OaPAC is a recently discovered blue-light-using flavin adenosine dinucleotide (BLUF) photoactivated adenylate cyclase from the cyanobacterium Oscillatoria acuminata that uses adenosine triphosphate and translates the light signal into the production of cyclic adenosine monophosphate. OaPAC is a homodimer of a 366-residue protein comprising an N-terminal BLUF domain and a C-terminal class III adenylyl cyclase (AC) domain. BLUF domains contain a flavin adenine dinucleotide (FAD) chromophore and are ubiquitous blue-light sensors that are found in bacteria and unicellular eukaryotes. The BLUF-regulated AC domain of OaPAC stimulates turnover of ATP up to 20-fold upon illumination.

Tyr6 plays a key role in the photoactivation mechanism of OaPAC and of BLUF domains in general. In PixD, the BLUF protein from Synechocystis, the equivalent mutation (Y8W) blocks the formation of the signalling state, whereas in OaPACBLUF a Y6W mutation was recently introduced to dissect the forward electron and proton transfer following blue-light excitation of the flavin. To investigate the structural role of this residue, we have replaced Tyr6 by a tryptophan (Y6W), a mutation which is expected to disturb the hydrogen-bond network [Fig. 1(b)] around the flavin and at the same time form a photoinactive enzyme (Lukacs et al., unpublished results). However, the most extensive change is the ∼85° rotation around the CG—CD bond of the Gln48 residue, with the distances of the amide nitrogen and carbonyl oxygen of the side chain of Gln48 to the N5 of the flavin changing from 3.3 and 3.1 Å to 3.1 and 4.0 Å, respectively. The isoalloxazine moiety also rotates a few degrees in the Y6W mutant and displays an average shift of 0.2 Å, and the side chain of Met92 rotates ∼20°, whereas no notable changes are observed for Trp90, which retains a Trpout orientation pointing away from the flavin as observed in the WT [Fig. 5(c)] and previously published WT OaPAC structures. In particular, in the Y6W OaPAC mutant the BLUF domain is closer to the AC domain compared with the analogous distance in WT OaPAC.

> GMKRLTWISKFSRPLSGDEIEAIGRISSQKNQQANVTGVLLCLDGIFFQILEGEAEKIDRIYERILADERHTDILCLKSEVEVQERMFPDWSMQTINLDENTDFLIRPIKVLLQTLTESHRILEKYTQPSIFKIISQGTNPLNIRPKAVEKIVFFSDIVSFSTFAEKLPVEEVVSVVNSYFSVCTAIITRQGGEVTKFIGDCVMAYFDGDCADQAIQASLDILMELEILRNSAPEGSPLRVLYSGIGLAKGKVIEGNIGSELKRDYTILGDAVNVAARLEALTRQLSQALVFSSEVKNSATKSWNFIWLTDSELKGKSESIDIYSIDNEMTRKSSGGLEIARNIGHYLERV> GSSDSDHRELIGDYSKAFLLQTVDGKHQDLKYISPETMVALLTGKFSNIVDKFVIVDCRYPYEYEGGHIKTAVNLPLERDAESFLLKSPIAPCSLDKRVILIFHSEFSSERGPRMCRFIRERDRAVNDYPSLYYPEMYI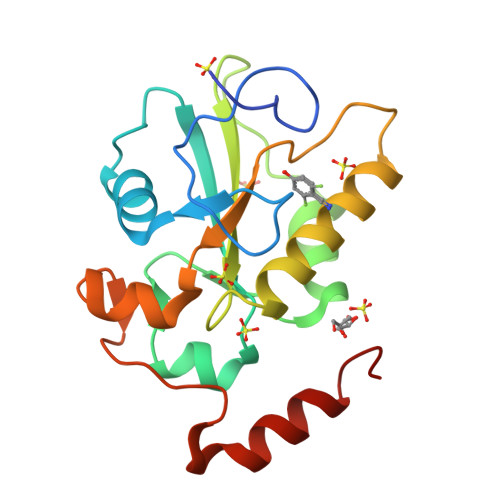LKGGYKEFFPQHPNFCEPQDYRPMNHEAFKDELKTFRLKTRSWA2-BENZYL-3-IODOPROPANOIC ACID | 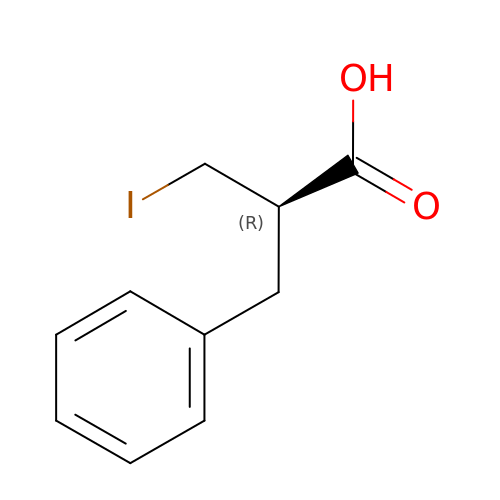C10 H11 I O2 | CRYXPGIJLMKFPX-VIFPVBQESA-N> RTFSYTLEDHTKQAFGVMNELRLSQQLCDVTLQVKYEDIPAAQFMAHKVVLASSSPVFKAM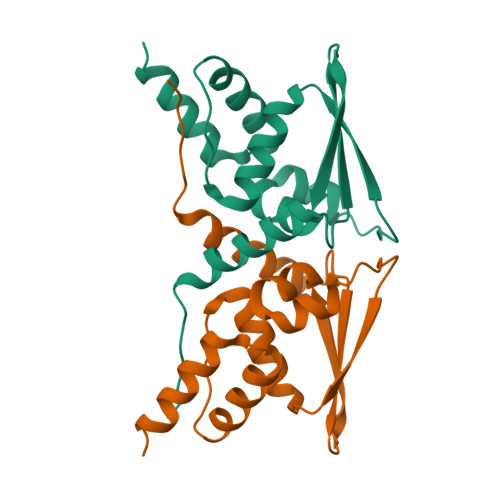FTNGLREQGMEVVSIEGIHPKVMERLIEFAYTASISVGEKCVLHVMNGAVMYQIDSVVRACADFLVQQL>[10x]MSTTIQYNSNYADYSISSYLREWANNF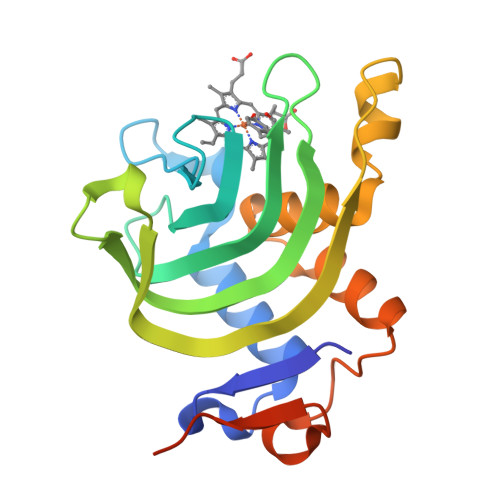GDIDQAPAETKDRGSFSGSSTLFSGTQYAIGSSHSNPEGMIAEGDLKYSFMPQHTFHGQIDTLQFGKDLATNAGGPSAGKHLEKIDITFNELDLSGEFDSGKSMTENHQGDMHKSVRGLMKGNPDPMLEVMKAKGINVDTAFKDLSIASQYPDSGYMSDAPMVDTV> MRGSHHHHHHGSKDAVNYELIWSEWVKEAPAKEAANREEAVQRMRDCLKNNKTELRLKILGLTTIPAYIPEQITTLILDNNELKSLPENLQGNIKTLYANSNQLTSIPATLPDTIQEMELSINRITELPERLPSALQSLDLFHNKISCLPENLPEELRYLSVYDNSIRTLPAHLPSEITHLNVQSNSLTALPETLPPGLKTLEAGENALTSLPASLPPELQVLDVSKNQITVLPETLPPTITTLDVSRNALTNLPENLPAALQIMQASRNNLVRLPESLPHFRGEGPQPTRIIVEYNPFSERTIQNMQRLMSSVDYQGPRVLFAMGDFSIVRVTRPLHQAVQGWLTSLEEEDVNQWRAFEAEANAAAFSGFLDYLGDTQNTRHPDFKEQVSAWLMRLAEDSALRETVFIIAMNATISCEDRVTLAYHQMQEATLVHDA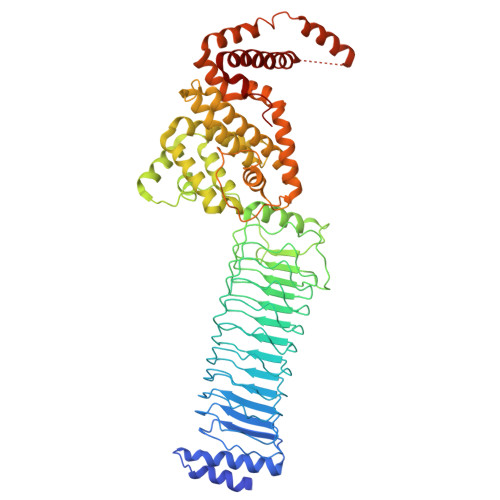ERGAFDSHLAELIMAGREIFRLEQIESLAREKVKRLFFIDEVEVFLGFQNQLRESLSLTTMTRDMRFYNVSGITESDLDEAEIRIKMAENRDFHKWFALWGPWHKVLERIAPEEWREMMAKRDECIETDEYQSRVNAELEDLRIADDSDAERTTEVQMDAERAIGIKIMEEINQTLFTEIMENILLKKEVSSLMSAYWR~{N}-[(1~{S})-1-(2,3-dihydro-1,4-benzodioxin-6-yl)ethyl]-2-methyl-pyridin-3-amine 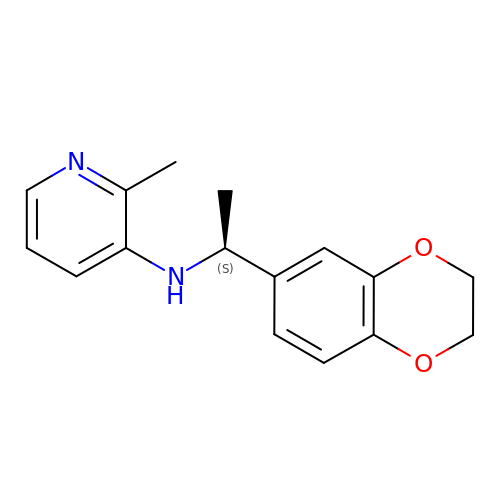| C16 H18 N2 O2 | UFPSUOFEQKCPHZ-NSHDSACASA-N1-[3-methyl-4-(piperidin-4-yloxy)-1-benzofuran-2-yl]-3-phenylpropan-1-one | C23 H25 N O3 | 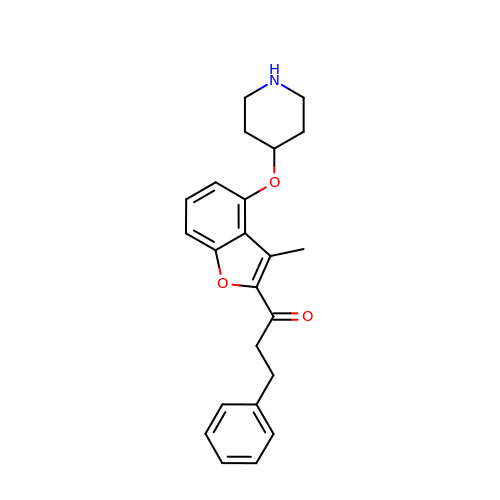ZUAGYVKWPGUWFU-UHFFFAOYSA-N SLX1 belongs to the GIY-YIG superfamily of nucleases. When bound to SLX4, SLX1 cleaves various branched DNA substrates near the branch point. Slx1 comprises two distinct domains: N-terminal GIY-YIG nuclease domain and C-terminal RING domain which binds two zinc ions. The CCD3 fragment of Slx4 bound between these two domains.

Crystals of Tt-Slx1–Slx4CCD3 that were grown in the presence of splayed-arm substrate belonged to the P21 space group. These crystals diffracted to a resolution of 2.7 Å. Unexpectedly, the DNA substrate, which was designed to adopt a splayed-arm conformation, was found to form a double-helical conformation, in which the two single-stranded overhangs were base-paired because of partial complementarity, forming a slightly distorted double helix with a 2-nt bulge and a G-A mismatch. The asymmetric unit of Tt-Slx1–Slx4CCD3-DNA crystals contained one DNA molecule that was bound by two protein molecules. The DNA-binding interface in each protein was identical and located on the side of the GIY-YIG domain at the edge of the central β-sheet. The protein bound the DNA backbone through basic amino acid side chains (R22, H23, R51, R54, K101 and R102) with a buried surface area of 637.3 Å2 in the better-organized protein–DNA interface. In the new Tt-Slx1–Slx4CCD3-DNA structure, the DNA was located away from the active site and occupied a markedly different position from the position that we predicted earlier. We designated this newly identified DNA-binding surface as site III. Therefore, upon DNA binding at site III, a part of this region that comprised residues 108–113 became ordered. We hypothesize that the ordering of this region is coupled to the proper assembly of the active site, which could serve as a safety latch mechanism (i.e. catalysis could only occur when DNA is bound at site III).

>MTVQCKPIPALYTVYVLRSTVRHASLYIGSTPNPPRRLKQHNGLVPGGAARTSRSSLRPWEMVALVSGFPSMVAALKFQWALTNPHLSVHIPSASRLTVATQTKANGRPQRPPRSLASVVANLHLLLRVPSFARWPLRVHFFRRDVFAAWEKWCAAASERLRPSLAVVTDFEGGSEGLAGAVVGGEEGRERGEGAPCWGIHALPLDYEPIKDYVAKGQEIFEFERQGACVVCREEMASGDGLQALCTNQGCDGVGHLSCWSRHFLKGAEADSILPVQGQCPKCGGEMEWGNMMKELTLRTRGQKEVEKLLKRKRRRATKKTANA[2x];>MEDTETSLVASPTDQQVSLFRYITQAVVTAPRAKDPANPSWHEKMLMYDPIILEDLTAWLNSGQLDRVGYDGEVAPGDVKKWCESKSVCCLWRVSLNGKERKRF[2x]>MTSTRLQKLRIRAPGCGTAEVTTSNAPSEEVTAVTTEVQGETEEKKKVLTTFTVLADMVQNVAGDKLVVESITRIGAEIHGYEPTPSDIVKAQDADLILYNGMNLERWFEQFLGNVKDVPSVVLTEGIEPIPIADG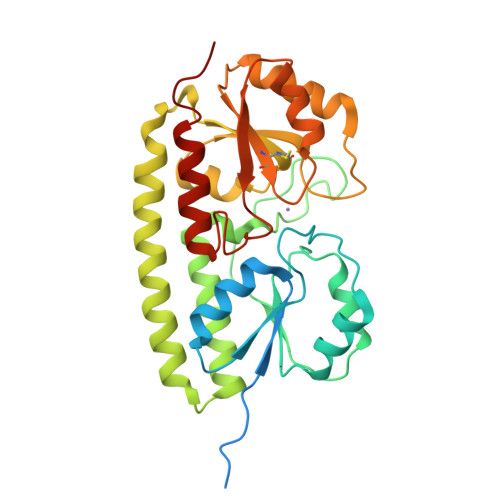PYTDKPNPHAWMSPRNALVYVENIRQAFVELDPDNAKYYNANAAVYSEQLKAIDRQLGADLEQVPANQRFLVSCEGAFSYLARDYGMEEIYMWPINAEQQFTPKQVQTVIEEVKTNNVPTIFCESTVSDKGQKQVAQATGARFGGNLYVDSLSTEEGPVPTFLDLLEYDARVITNGLLAGTNAQQ[3x]> METDLNSQDRKDLDKFIKFFALKTVQVIVQARLGEKICTRSSSSPTGSDWFNLAIKDIPEVTHEAKKALAGQLPAVGRSMCVEISLKTSEGDSMELEIWCLEMNEKCDKEIKVSYTVYNRLSLLLKSLLAITRVTPAYRLSRKQGHEYVILYRIYFGEVQLSGLGEGFQTVRVGTVGTPVGTITLSCAYR;> MNCRSEVLEVSVEGRQVEEAMLAVLHTVLLHRSTGKFHYAAAGTYSIGTVGTQDVDCDFIDFTYVRVSSEELDRALRKVVGEFKDALRNSGGDGLGQMSLEFYQKKKSRWPFSDECIPWEVWTVKVHVVALATEQERQICREKV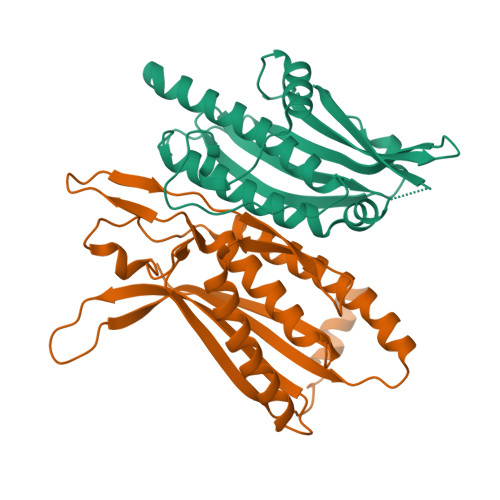GEKLCEKIINIVEVMNRHEYLPKMPTQSEVDNVFDTGLRDVQPYLYKISFQITDALGTSVTTTMRRLIKDTLAL>GSHMSEPTSSSSLDITSNCIIETPLQPSDFLPKSANLFPKFPERISVDSWELWEFDTFDTNGSVAFGCSLYRDARGVEQGGFHAEVNALWPDGTHWGETLYFAVSEVVENSDGTTGGKWLSKDGGSITFHIASDYTAAALDFNVPGKVSGTMELRNHANVSPTSNLPASDAEAQLCPGVYYTFPMGPVATSVTATFSSVGANGESRELFISSGYGGMVRGWSARPWPTFMNDAYYVVAQVGPYMLQILRTLGSVFVQHKPFAVARLYLDGSLVSAANTVVGDELTAHADDVKGDAVRLTKVQPDEKSQGLSGKFRDGNVGYVLEFAKKDSEHGWTFQISHKRAVWSEPTSAPGPDGTGKSGWIEAISGGA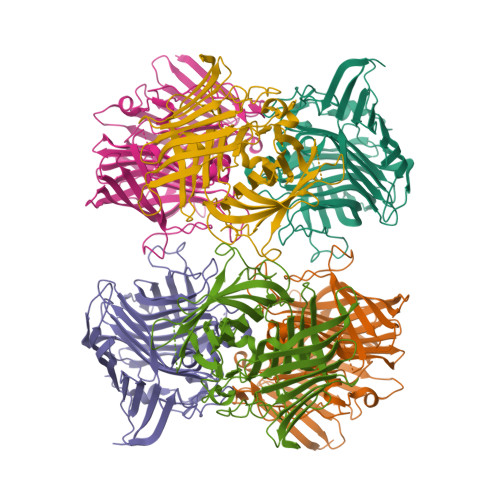KGENYEGHGFGGQLQIPVP[6x]>GPPVVEEDDVVGFDDEAQTVIDRLLEGSGDLEVIPVVGMPGLGKTTLATKIFKHPKIEYEFFTRLWLYVSQSYKTRELYLNIISKFTGNTKHCRDMSEKDLALKVQEILEEGGKYLIVLDDVWSTDAWDRIKIAFPKNDKGNRVLLTTRDHRVARYCNRSPHDLKFLTDEESWILLEKRAFHKAKCLPELETNGKSIARKCKGLPLAIVVIAGALIGKSKTIKEWEQVDQSVGEHFINRDQPNSCDKLVRMSYDVLPYDWKACFLYFGTFPRGYLIPARKLIRLWIAEGFIQYRGDLSPECKAEEYLNELVNRNLVMVMQRTVDGQIKTCRV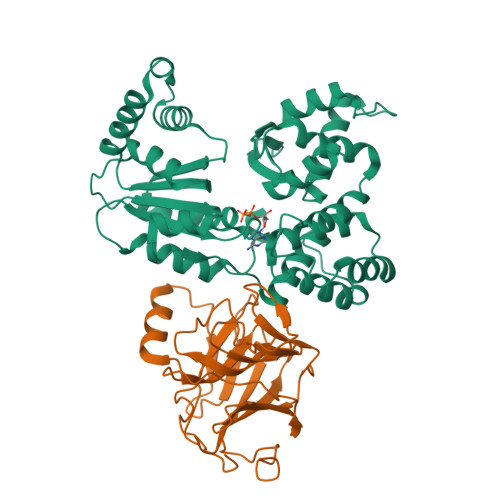HDMLYEFCWQEATTE[2x];>[2x]GPSPKANAKLEKVPSGNAESTPVLTLQNRWAYSARDEKLAWDSAARDEKLELTEPAGLIVQFIGENSKHRSVRAKLPIPKGNSGIFYYEVTISGDGDAIYIGLATEQMPLRDTHVGYNEGTYGYGSSGKFWGHEVGGCSHWGNERPYIDGQPKFDRNNIIGCGVNLKTRQIIYTHNGRPLETTGLLVAESAAELYPCVSLFTSGNEIEANFGTKPFKFNIAEGI> MPINRPNLNLNIPPLNIVAAYDGAEIPSTNKHLKNNFNSLHNQMRKMPVSHFKEALDVPDYSGMRQSGFFAMSQGFQLNNHGYDVFIHARRESPQSQGKFAGDKFHISVLRDMVPQAFQALSGLLFSEDSPVDKWAVTDME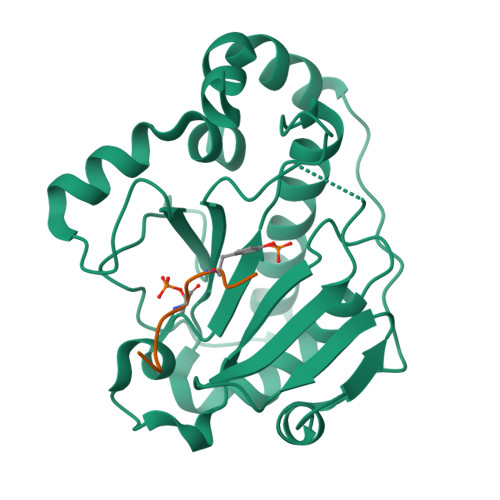KVVQQARVSLGAQFTLYIKPDQENSQYSASFLHKTRQFIECLESRLSENGVISGQCPESDVHPENWKYLSYRNELRSGRDGGEMQRQALREEPFYRLMTE;> QYFMTEYVA>[4x]MSIKEQTLMTPYLQFDRNQWAALRDSVPMTL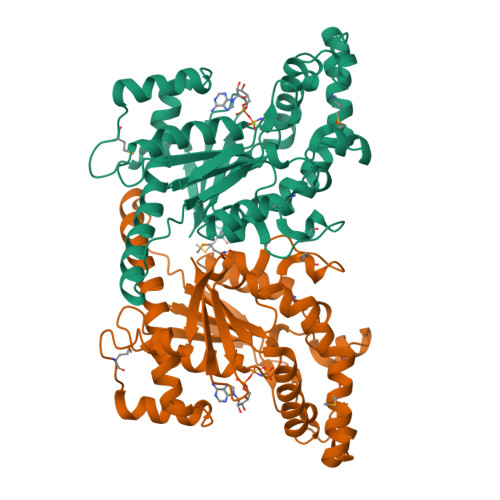SEDEIARLKGINEDLSLEEVAEIYLPLSRLLNFYISSNLRRQAVLEQFLGTNGQRIPYIISIAGSVAVGKSTTARVLQALLSRWPEHRRVELITTDGFLHPNQVLKERGLMKKKGFPESYDMHRLVKFVSDLKSGVPNVTAPVYSHLIYDVIPDGDKTVVQPDILILEGLNVLQSGMDYPHDPHHVFVSDFVDFSIYVDAPEDLLQTWYINRFLKFREGAFTDPDSYFHNYAKLTKEEAIKTAMTLWKEINWLNLKQNILPTRERASLILTKSANHAVEEVRLRK> MGSALSPTQSPSEFIAELARCAQPIAQANDLYASVMMAQAIVESGWGASTLSKAPNYNLFGIKGSYNGQSVYMDTWEYLNG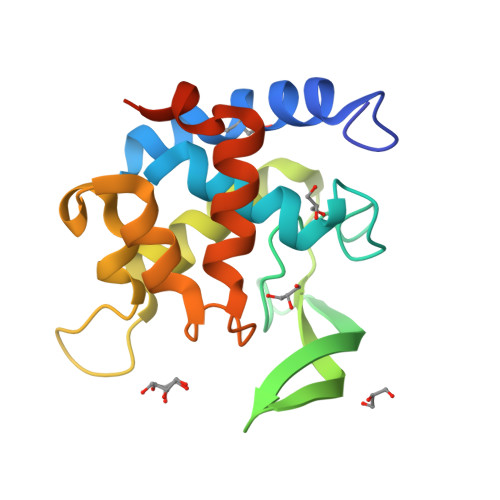KWLVKKEPFRKYPSYMESFQDNAHVLKTTSFQAGVYYYAGAWKSNTSSYRDATAWLTGRYATDPSYNAKLNNVITAYNLTQYDTPSSGSHHHHHH>MKQYLELMQKVLDEGTQKNDRTGTGTLSIFGHQMRFNLQDGFPLVTTQRCHLRSIIHELLWFLQGDTNIAYLHENNVTIWDEWADENGDLGPVYGKQWRAWPTPDGRHIDQITTVLNQLKNDPDSRRIIVSAWNVGELDKMALAPCHAFFQFYVADGKLSCQLYQRSCDVFLGLPFNIASYALLVHMMAQQCDLEVGDFVWTGGDTHLYSNHMDQTHLQLSREPRPLPKLIIKRKPESIFDYRFEDFEIEGYDPHPGIKAP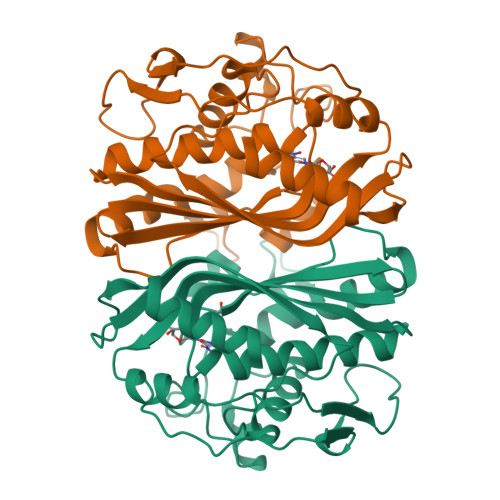VAI[2x]> ASAPIGSAISRNNWAVTCDSAQSGNECNKAIDGNKDTFWHTFYGANGDPKPPHTYTIDMKTTQNVNGLSMLPRQDGNQNGWIGRHEVYLSSDGTNWGSPVASGSWFADSTTKYSNFETRPARYVRLVAITEANGQPWTSIAEINVFQASSYTAPQPGLGRWGPTIDLPIVPAAAAIEPTSGRVLMWSSYRNDAFGGSPGGITLTSSWDPSTGIVSDRTVTVTKHDMFCPGI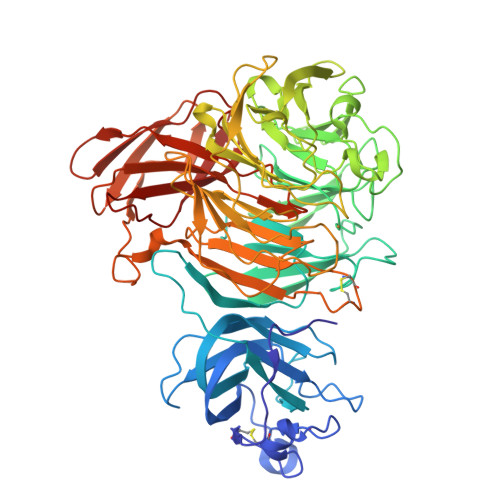SMDGNGQIVVTGGNDAKKTSLYDSSSDSWIPGPDMQVARGYQSSATMSDGRVFTIGGSFSGGVFEKNGEVYSPSSKTWTSLPNAKVNPMLTADKQGLYRSDNHAWLFGWKKGSVFQAGPSTAMNWYYTSGSGDVKSAGKRQSNRGVAPDAMCGNAVMYDAVKGKILTFGGSPDYQDSDATTNAHIITLGEPGTSPNTVFASNGLYFARTFHTSVVLPDGSTFITGGQRRGIPFEDSTPVFTPEIYVPEQDTFYKQNPNSIVRVYHSISLLLPDGRVFNGGGGLCGDCTTNHFDAQIFTPNYLYNSNGNLATRPKITRTSTQSVKVGGRITISTDSSISKASLIRYGTATHTVNTDQRRIPLTLTNNGGNSYSFQVPSDSGVALPGYWMLFVMNSAGVPSVASTIRVTQ>[2x]QGPGGGGSVTCPGGQSTSNSQCCVWFDVLDDLQTNFYQGSKCESPVRKSLRIAFHDAIGFSPALTAAGQFGGGGADGSIIAHSNIELAFPANGGLTDTVEALRAVGINHGVSFGDLIQFAAAVGMSNCPGSPRLEFLTGRSNSSQPSPPSLIPGPGNTVTAILDRFGDAGFSPDEVVDLLAAHS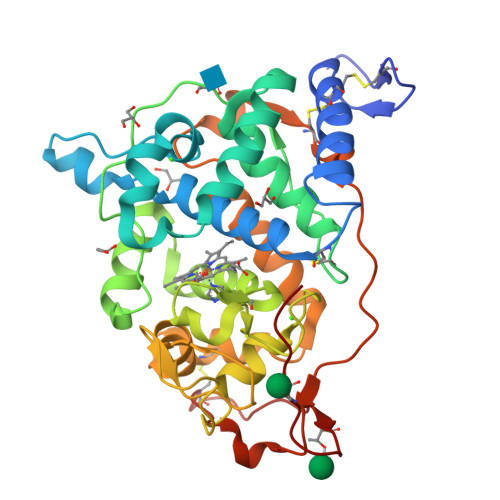LASQEGLNSAIFRSPLDSTPQVFDTQFYIETLLKGTTQPGPSLGFAEELSPFPGGFRIRSDALLARDSRTACRWQSMTSSNEVMGQRFRAAMAKMSVLGFDRNALTDCSDVIPSAVSNNAAPVIPGGLTVDDIEVSCPSEPFPEIATASGPLPSLAPAP> GPHMTVFHDKENF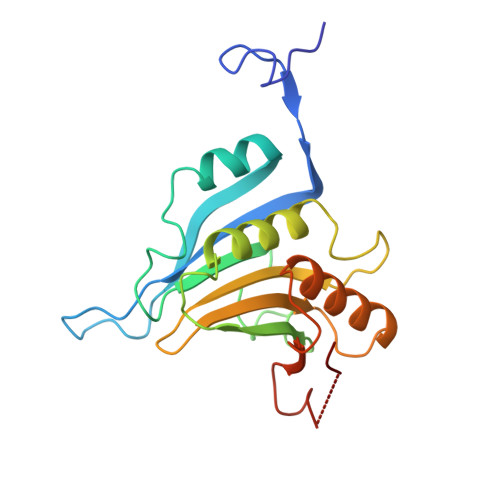NVKHPLSCRWTLWFTKPASGKGDNWNDLLKKVITFESVEEFWGIYNNIAPVSELAVKSDYHLFKEGVRPEWEDPQNKHGGKWAYQFKDKRSVNIDELWLHTMLAAIGETLEDEEDGEVMGVVVNVRKGFYRIGVWTRTTEKSKEILMNIGRRLKEVLKLPPNEMVEFSGHTEAAQAGSTRAKARMVV>GPLGSDRSPTDKELVSQAKALCRDYINSRLIRAGVSWSKPEHNTPVPGGKLAEVSAILLRLGDELEYIRPNVYRNIARQLNISLHSETVVTDAFLAVAAQIFTAGITWGKVVSLYAVAAGLAVDCVRHAQPA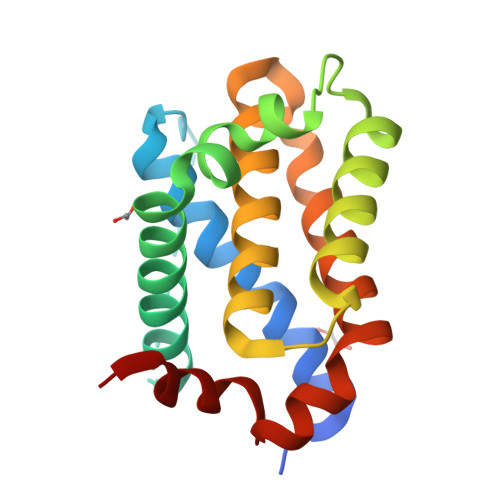MVHTIVDCLGEFVRKTLVTWLKRRGGWADITKCVVS[2x]>[2x]SEILRYLMDPDTFTSNFNNDPLVLRRRQTYLCYEVERLDNGTSVKMDQHMGFLC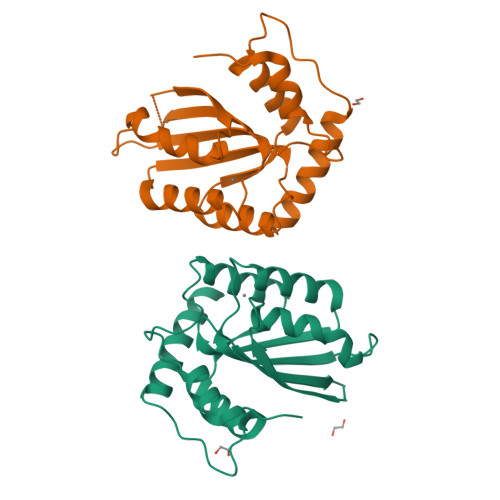NESGRHAELRFLDLVPSLQLDPAQIYRVTWFISWSPCFSWGCAGEVRAFLQENTHVRLRIKAARIYDYDPLYKEALQMLRDAGAQVSIMTYDEFEYCWDTFVYRQGCPFQPWDGLEEHSQALSGRLRAILQ Patatin is a soluble 40 kDa non-specific plant lipase that is expressed extensively in the tubers of potatoes and other members of the nightshade family. Previously, the crystal structure of a recombinant patatin isoform, patatin-17 (pat17), derived from the tubers of heartleaf nightshade (Solanum cardiophyllum), has shown this protein to have a modified α/β hydrolase fold containing a central 6-stranded β-sheet sandwiched by 9 α-helices along with a catalytic center composed of a Ser77-Asp215 dyad. This fold and active site configuration is reminiscent of the human cytosolic phospholipase A2 family of enzymes, but it is distinct from the traditional Ser-His-Asp/Glu catalytic triads found in serine proteases and esterases such as chymotrypsin and acetylcholinesterase (AChE), respectively. Recently, interest in patatin and its homologues has been heightened by the discovery that a diverse group of mammalian lipases, termed the patatin-like phospholipase domain containing proteins (PNPLAs), encompass catalytic domains with sequence similarity to patatin.

Overall, our structure of native (non-derivatized) pat17 is similar to the SeMet-derivatized structure described previously by Rydel et al. (RMSD  = 0.27 Å). Pat17 purified and crystallized as a monomer in the asymmetric unit. In agreement with results presented by Rydel et al., pat17 consists of 8 β-strands and 9 α-helices arranged in a modified α/β hydrolase fold with a central 6-stranded β-sheet consisting of five parallel and one anti-parallel β-strands sandwiched by 2 α-helices in the front and 7 α-helices in the back. The catalytic Ser77 is located on a loop between β2 and α2 (termed the nucleophilic elbow) that contains the classic G-X-S-X-G lipase consensus sequence motif. Ser77 lies adjacent to Asp215 creating a catalytic dyad defined by Rydel et al.. In contrast, the catalytic dyad of pat17 functions with Asp215 acting as the general base that activates the catalytic Ser77 residue. The catalytic dyad of pat17 sits at the bottom of a large chamber (153.6 Å3 calculated using VOIDOO) lined with the following residues: Gly36, Gly37, Gly38, Ile39, Ser77, Thr78, Leu81, Phe105, Tyr106, Gly110, Phe114, Phe194, and Asp215. Two portals were found to flank helix 7 (α7) with the first portal (portal) being 16 Å in length and lined with the following residues: Ala190, Pro191, Ala 217, Val218, Gln288, Thr291 and Asp292. The second portal (portal) is 15.2 Å in length and is lined with the following residues: Arg40, Gly261, Thr262, Lys289, Asp292, Ala293, Gln320, Leu324, Thr329 and Met331. Comparison of the DFP-aged structure of pat17 and the MAFP-inhibited structure to the native pat17 structure yielded Cα backbone RMSD values of 0.19 Å (DFP- aged vs. native) and 0.12 Å (MAFP-inhibited vs. native).

> MHHHHHHAMAQLGEMVTVLSIDGGGIRGIIPATILEFLEGQLQEMDNNADARLADYFDVIGGTSTGGLLTAMISTPNENNRPFAAAKEIVPFYFEHGPQIFNPSGQILGPKYDGKYLMQVLQEKLGETRVHQALTEVVISSFDIKTNKPVIFTKSNLANSPELDAKMYDISYSTAAAPTYFPPHYFVTNTSNGDEYEFNLVDGAVATVADPALLSISVATRLAQKDPAFASIRSLNYKKMLLLSLGTGTTSEFDKTYTAKEAATWTAVHWMLVIQKMTDAASSYMTDYYLSTAFQALDSKNNYLRVQENALTGTTTEMDDASEANMELLVQVGENLLKKPVSEDNPETYEEALKRFAKLLSDRKKLRANKASY> MKKTAIAIAVALAGFATVAQASPDTSVDNKVNFSTDVIYQIVTDRFADGDRTNNPAGDAFSGDRSNLKLYFGGDWQGIIDKINDGYLTGMGVTALWISQPVENITSVIKYSGVNNTSYHGYWARDFKQTNDAFGDFADFQNLIDTAHAHNIKVVIDFAPNHTSPADRDNPGFAENGALYDNGSLLGAYSNDTAGLFHHNGGTDFSTIEDGIYKNLYDLADINHNNNAMDAYFKSAIDLWLGMGVDGIRFDAVKHMPFGWQKSFVSSIYGGDHPVFTFGEWYLGADQTDGDNIKFANESGMNLLDFEYAQEVREVFRDKTETMKDLYEVLASTESQYDYINNMVTFIDNHDMDRFQVAGSGTRATEQALALTLTSRGVPAIYYGTEQYMTGDGDPNNRAMMTSFNTGTTAYKVIQALAPLRKSNPAIAYGTTTERWVNNDVLIIERKFGSSAALVAINRNSSAAYPISGLLSSLPAGTYSDVLNGLLNGNSITVGSGGAVTNFTLAAGGTAVWQYTAPETSPAIGNVGPTMGQPGNIVTIDGRGFGGTAGTVYFGTTAVTGSGIVSWEDTQIKAVIPKVAAGKTGVSVKTSSGTASNTFKSFNVLTGDQVTVRFLVNQANTNYGTDVYLVGNAAELGSWDPNKAIGPMYNQVIAKYPSWYYDVSVPAGTKLDFKFI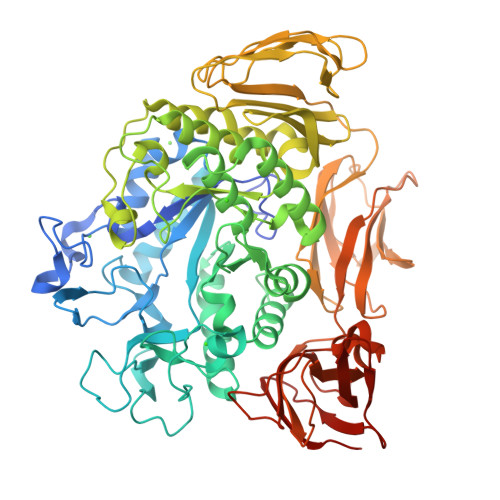KKGGGTVTWEGGGNHTYTTPASGVGTVTVDWQN> STPDQSTAYMQGTAQADSAFYLQQMQQSSDDTRINWQLLAIRALVKEGKTGQAVELFNQLPQELNDAQRREKTLLAVEIKLAQKDFAGAQNLLAKITPADLEQNQQARYWQAKIDASQGRPSIDLLRALIAQEP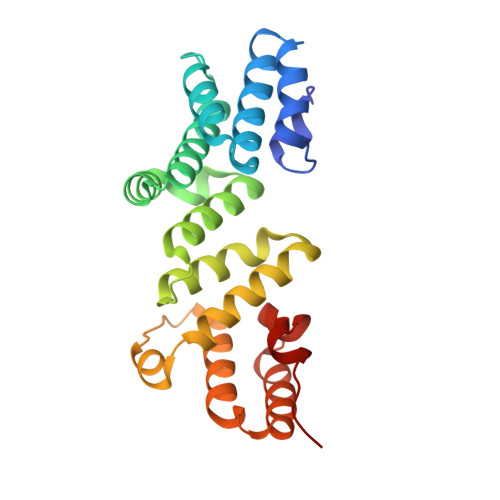LLGAKEKQQNIDATWQALSSMTQEQANTLVINADENILQGWLDLQRVWFDNRNDPDMMKAGIADWQKRYPNNPGAKMLPTQLVNVKAFK>[2x]SKWPEPVFGRLVSPGFPEKYGNHQDRSWTLTAPPGFRLRLYFTHFNLELSYRCEYDFVKLTSGTKVLATLCGQESTDTERAPGNDTFYSLGPSLKVTFHSDYSNEKPFTGFEAFYAAEDVDECRTSLGDSVP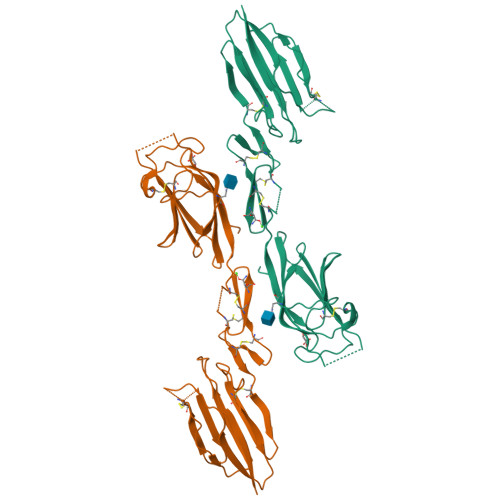CDHYCHNYLGGYYCSCRVGYILHQNKHTCSALCSGQVFTGRSGFLSSPEYPQPYPKLSSCAYNIRLEEGFSITLDFVESFDVEMHPEAQCPYDSLKIQTDKREYGPFCGKTLPPRIETDSNKVTITFTTDESGNHTGWKIHYTSTAQPHHHHHH>SKINVNVENVSGVQGFLFHTDGKESYGHRAFINGVEIGIKDIETVQGFQQIIPSI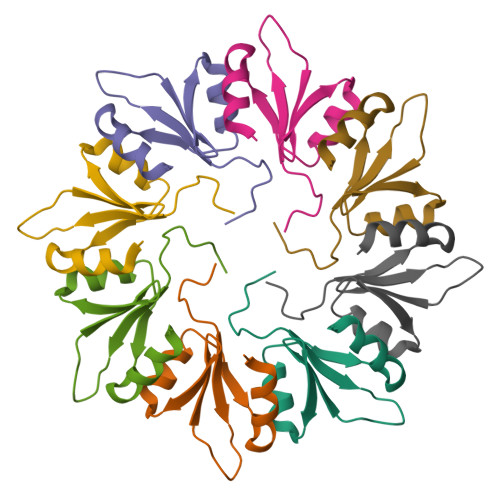NISKSDVEAIRKAMKK[2x]>[2x]MEPQ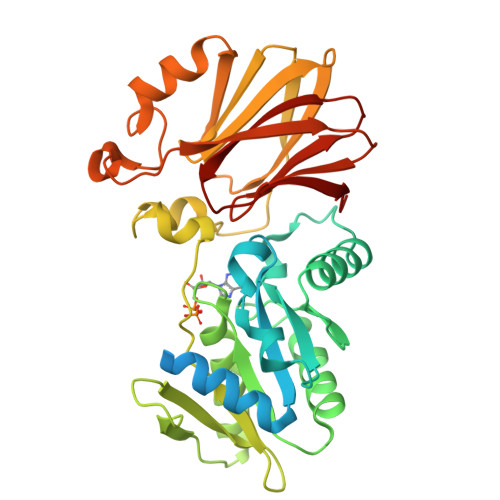LRCIGCGAAIQFENPKNAGYAPKSVLEKDAEEVICQRCFRLKHYNEVQDVPLDDDDFLSMLHRIGESKALVVNIVDIFDFNGSFIPGLPRFAADNPILLVGNKADLLPRSVKYPKLLRWMRRMAEELGLCPVDVCLVSAAKGIGMAKVMEAINRYREGGDVYVVGCTNVGKSTFINRIIEEATGKGNVITTSYFPGTTLDMIEIPLESGATLYDTPGIINHHQMAHFVDARDLKIITPKREIHPRVYQLNEGQTLFFGGLARLDYIKGGRRSFVCYMANELTVHRTKLEKADSLYANQLGELLSPPSKRYAAEFPPLVPRSLSVKERKTDIVFSGLGWVTCNDPGAQLVVHAPKGVDVFIRQSLI> MGHHHHHHRINHNIAALNTLNRLSSNNSASQKNMEKLSSGLRINRAGDDAAGLAISEKMRGQIRGLEMASKNSQDGISLIQTAEGALTETHAILQRVRE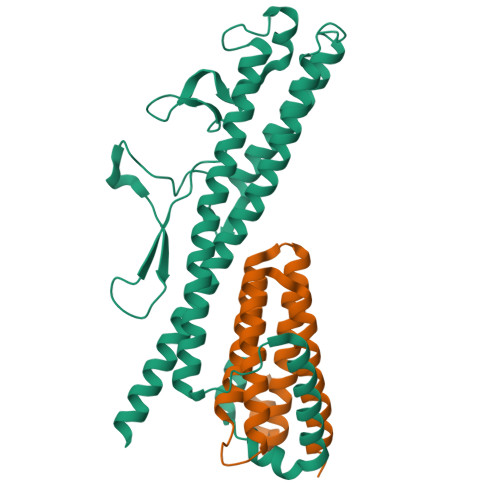LVVQAGNTGTQDKATDLQSIQDEISALTDEIDGISNRTEFNGKKLLDGTYKVDTATPANQKNLVFQIGANATQQISVNIEDMGADALGIKEADGSIAALHSVNDLDVTKFADNAADTADIGFDAQLKVVDEAINQVSSQRAKLGAVQNRLEHTINNLSASGENLTAAESRIRDVDMAKEMSEFTKNNILSQASQAMLAQANQQPQNVLQLLR;> MAIQNPYTAYQQNSVNTATPGELTLMLYNGCLKFIRLAAQAIENDDMERKNENLIKAQNIIQELNFTLNRNIELSASMGAMYDYMYRRLVQANIKNDTGMLAEVEGYVTDFRDAWKQAIQSERKDRHGSGGIA9H-purin-2-amine | C5 H5 N5 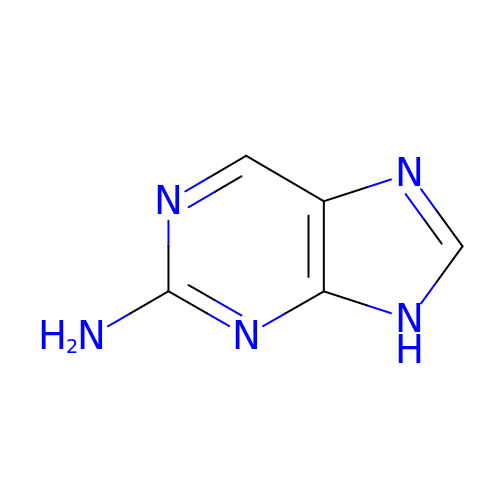| MWBWWFOAEOYUST-UHFFFAOYSA-N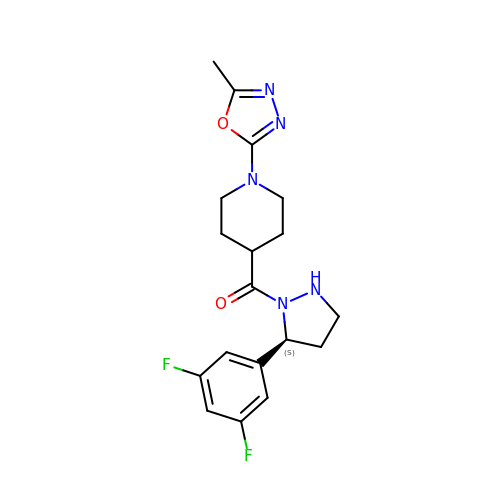[(5~{S})-5-[3,5-bis(fluoranyl)phenyl]pyrazolidin-1-yl]-[1-(5-methyl-1,3,4-oxadiazol-2-yl)piperidin-4-yl]methanone | C18 H21 F2 N5 O2 | KYFXWICBRBBWQQ-INIZCTEOSA-N> AE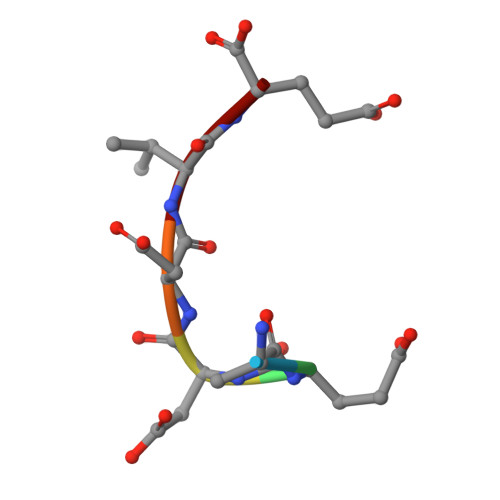DDVE BIS[5-CHLORO-1H-INDOL-2-YL-CARBONYL-AMINOETHYL]-ETHYLENE 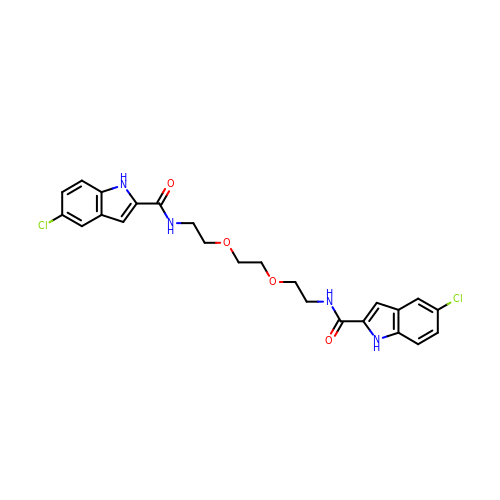GLYCOL | C24 H24 Cl2 N4 O4 | MWWXABBBAPKJDX-UHFFFAOYSA-N(2-oxopropyl)phosphonic acid | C3 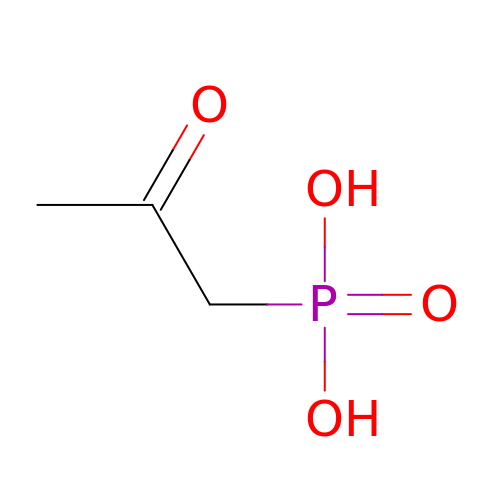H7 O4 P | DVSHXLWNRCEDCW-UHFFFAOYSA-N> CLAVPGKVIEVNGPVAVVDFG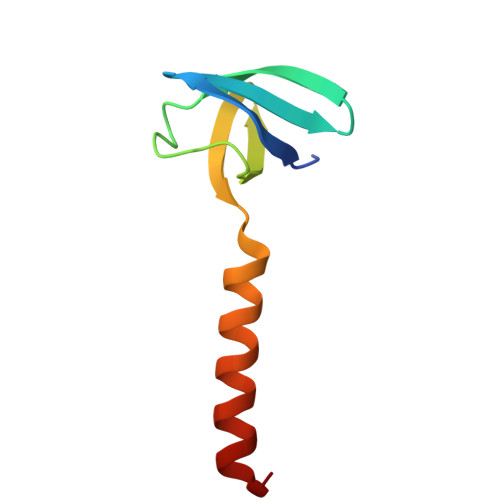GVKREVRLDLMPDTKPGDWVIVHTGFAIEKLDEKKAMEILEAWAEVEKAMEGF> MPPNSRIFLVISKYTPESVLRERFSPFGDIQDIW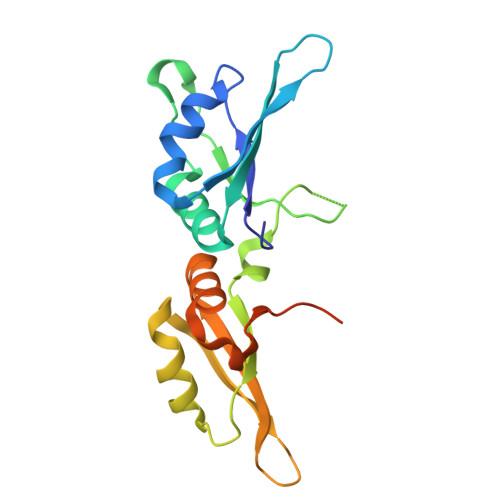VVRDKHTKESKGIAFVKFARSSQACRAMEEMHGQCLGPNDTKPIKVFIAQSRSSGSHRDVEDEELTRIFVMIPKSYTEEDLREKFKVYGDIEYCSIIKNKVTGESKGLGYVRYLKPSQAAQAIENCDRSFRAILAEPKNKASESSEQLEHHHHHH> XQQVHVLSLDQIRAIRNTNE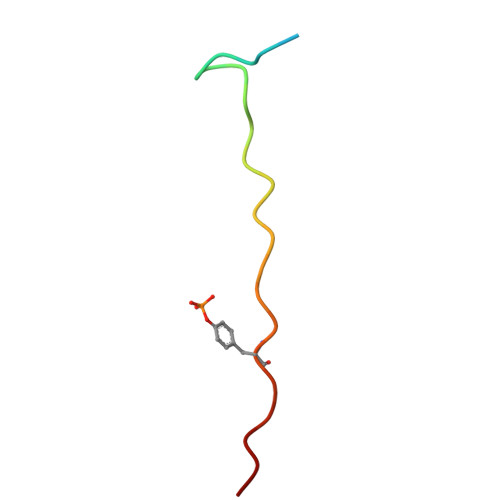YTEGPT(3S)-4-(5-chloro-1H-benzimidazol-2-yl)-3-(4-chlorophenyl)butanoic acid | C17 H14 Cl2 N2 O2 | 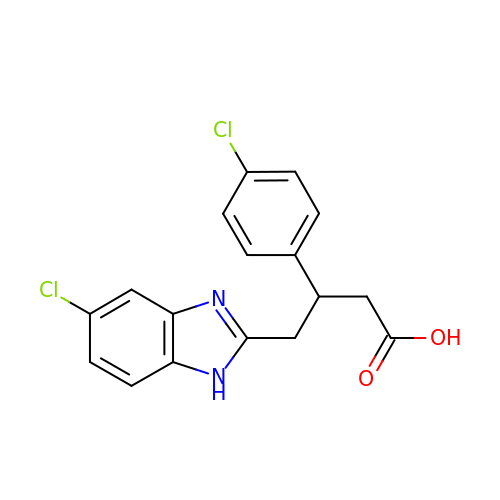MOXSMEYUODNXTB-UHFFFAOYSA-N>[2x]XSLSDKDKAAVRALWSKIGKSSDAIGNDALSRMIVVYPQTKIYFSHWPDVTPGSPNIKAHGKKVMGGIALAVSKIDDLKTGLMELSEQHAYKLRVDPSNFKILNHCILVVISTMFPKEFTPEAHVSLDKFLSGVALALAERYR;>[2x]VEWTDKERSIISDIFSHMDYDDIGPKALSRCLVVYPWTQRYFSGFGNLYNAEGIMSNANVA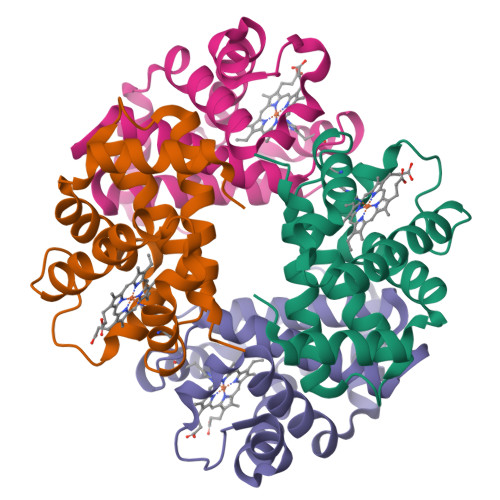AHGIKVLHGLDRGMKNMDNIADAYTDLSTLHSEKLHVDPDNFKLLSDCITIVLAAKMGHAFTAETQGAFQKFLAAVVSALGKQYH> MRGSHHHHHHGSMQEVTMWGDSHGVAPNQVRRTLVKVALSESLPPGAKQIRIGFSLPKETEEKVTALYLLVSDSLAVRDLPDYKGRVSYDSFPISKEDRTTALSADSVAGRRFFYLAADIGPVASFSRSDTLTARVEEVAVDGRPLPLKELSPASRRLYRGYEALFVPGDGGSRNYRIPAILKTANGTLIAMADRRKYNQTALPEDIDIVMRRSTDGGKSWSDPRIIVQGEGRNHGFGDVALVQTQAGKLLMIFVGGVGLWQSTPDRPQRTYISESRDEGLTWSPPRDITHFIFGKDCADPGRSRWLASFCASGQGLVLPSGRITFVAAIRESGQEYVLNNYVLYSDDEGDTWQLSDCAYRRGDEAKLSLMPDGRVLMSIRNQGRQESRQRFFALSSDDGLTWERAKQFEGIHDPGCNGAMLQVKRNGRDQVLHSLPLGPDGRRDGAVYLFDHVSGRWSAPVVVNSGSSAYSDMTLLADGTIGYFVEEGDEISLVFIRFVLDDLFDVRQ

The oral bacterium Porphyromonas gingivalis, a “keystone” pathogen of periodontitis, produces a dual domain sialidase (PG0352). Biochemical analyses reveal that PG0352 can desialylate human serum and complement factors and thus protect bacteria from serum killing. Structural analyses show that PG0352 contains a N-terminal carbohydrate-binding module (CBM) and a C-terminal sialidase domain that exhibits a canonical six-bladed β-propeller sialidase fold with each blade composed of 3–4 antiparallel β-strands. Structural and functional analyses further demonstrate that the CBM binds to carbohydrates and serum glycoproteins.

To probe how PG0352 interacts with native glycans, we engineered a D219A mutation in PG0352 to inhibit the ability of the enzyme to hydrolyze the glycosidic bond. We subsequently co-crystallized D219A PG0352 with 3’-sialyllactose (3’-SL) and 6’-sialyllactose (6’-SL) and solved their structures utilizing molecular replacement methods to 1.42Å and 1.41Å, respectively. The overall architectures of the CBM and sialidase domains are completely conserved in the structures. In each structure, the sugar ring of the sialic acid moiety adopts a distorted-boat conformation, with shifts in the positions of the O2, O6, and C7 hydroxyl group of ~0.5Å when compared to DANA, due to the D219A substitution. Otherwise, the residues and interactions involved in the binding of the terminal sialic acid moiety in the PG0352:3’-SL and PG0352:6’-SL structures are essentially identical to that observed for the binding of Neu5Ac in the PG0352:Neu5Ac structure. Three additional ordered water molecules are observed in the active site. One ordered water occupies the space vacated by the Asp-219 side chain, coordinating the O2 atom to the main chain amide of Ala-219 and the side chain of Arg-194. The other two ordered waters are part of an interaction network that connects the carboxylate of sialic acid to the side chains of Trp-278, Arg-398, and Gln-400. There is no clear electron density within the PG0352:3’-SL or PG0352:6’-SL crystal structures to facilitate the modeling of the galactose or glucose moieties. The absence of electron density for these moieties suggests that there are no specific interactions between PG0352 and glycan substrates at the active site, except for the terminal sialic acid.Cyclodipeptide synthases (CDPSs) use aminoacylated tRNA (aa-tRNA) substrates to form peptide bonds between two amino acids yielding a cyclic dipeptide product (CDP). ParaCDPS from Parabacteroides sp. 20_3 (GenBank: EFK64745.1) produces cyclo(His-Phe)8 whilst ParcuCDPS from Parcubacteria bacterium RAAC4_OD1_1 (GenBank: ETB63777.1) can synthesise both cyclo(His-Glu) and cyclo(His-Pro)9. ParcuCDPS belongs to the XYP sub-group of the CDPS family, characterised by the presence of 3 residues: X40 where X is a non-conserved residue, Y202, and P203 (numbering respective to AlbC). ParcuCDPS displays a Rossman-fold common throughout the CDPS family.

We solved the crystal structure of ParcuCDPS at a resolution of 1.90 Å (9 residues out of the total 230 were not traceable), uncovering unique characteristics of histidine substrate selection. The structure was solved by iodide SAD phasing after extensive failed trials of molecular replacement, suggesting substantial deviation from previously determined CDPS structures. The active site includes the four conserved residues previously identified: S26, Y167, E171 and Y191. Additionally, we hypothesised D58 was acting as a potential active site residue, within hydrogen bond distance from the catalytic serine (S26), which could be important for S26 to act as a nucleophile. Moreover, the side chain of the predicted catalytically important Y167 points away from the active site, removing the conventional hydrogen bonding network seen in other CDPSs. ParcuCDPS structure diverges from the common fold in helix α3 and beta-strand β3, where these regions change direction. In the common CDPS fold helix α3 and α4 exist as a single continuous helix whereas, in ParcuCDPS a flexible glycine residue (G84) provides a significant bend and change of direction, splitting the helix into two. β3 holds another important deviation seen in ParcuCDPS’ structure, as it changes direction (compared to common CDPS fold) at I56 to divide the active site pocket. This structural change of β3 facilitates the placement of D58 into H-bonding distance of the active site S26. CASTp38 was used to investigate the pocket volume of ParcuCDPS and highlighted pocket residues which are unique. P1 (shown in blue in Fig. 4c) is found deeper within the enzyme and is smaller and more restricted in size than P2 which sits at the solvent-accessible edge of the CDPS. From these calculations, P1 is predicted to be mostly neutral apart from Tyr55 and Glu174 which form a negatively charged microenvironment, while P2 is predicted to be mostly lined by positively charged residues.

> MELHQIRGCHKNDIELKKYNIGVAISLGNKWFSIDNIEKLVKWSLLHTKEYVIIYIADSIHGINLSVRNKLSDSHAEEVAIRYGRNLFIKIKERVSLSFSQDEQAKIIYATWSDIADSKYKEKVKYLYNLYDKNINFKNYIENFVKEWVSKEKRTFNNNEINKFGRYILEELPELMVQVKARGVLFEAYVYPYKTRITEFVGLLQKGEIFPEIKTNILDNHPKIFLEVRE> HRPEGLEQLEAQTNFTKRELQVLYRGFKNECPSGVVNEETFKQIYAQFFPHGDASTYAHYLFNAFDTTQTGSVKFEDFVTALSILLRGTVHEKLRWTFNLYDINKDG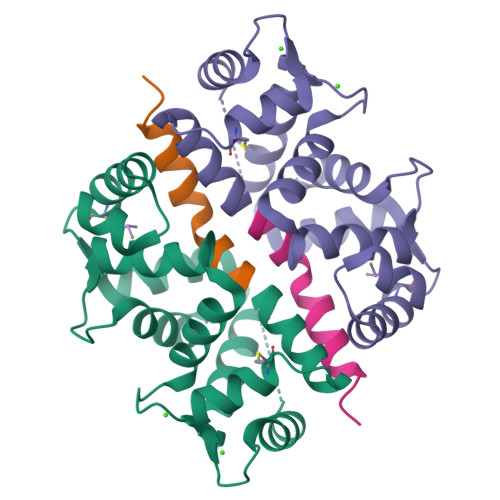YINKEEMMDIVKAIYDMMGKYTYPVLKEDTPRQHVDVFFQKMDKNKDGIVTLDEFLESCQEDDNIMRSLQLFQNVM;> MAAGVAAWLPFARAAAIGWMPVASGPMPAP> GSPEFME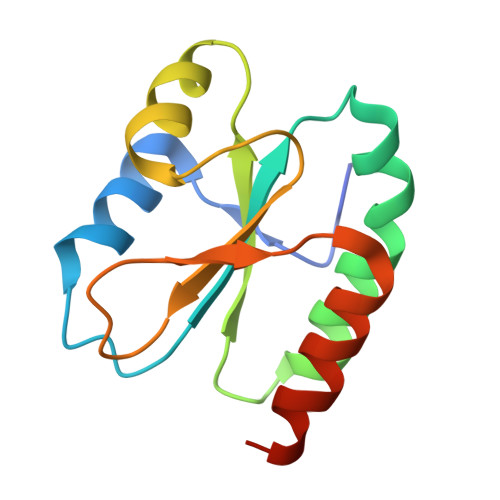NLVTLSRQGIENLMKLENRKEPWIVVLYAPWCPFCQAMEASYDELADKLAGSGIKVAKFRADGDQKEFAKQELQLGSFPTILVFPKNSSRPIKYPSEKRDVESLTSFLLEHHHHHH Type-IIa receptor protein tyrosine phosphatases (RPTPs) and neurexins are the two major presynaptic organizers. In mammals, the type-IIa RPTPs have three members, PTPδ, PTPσ, and LAR. These members possess a large extracellular domain (ECD) consisting of three immunoglobulin-like (Ig) domains and four to eight fibronectin type-III (Fn) domains, followed by a single transmembrane helix and a cytoplasmic domain harboring two protein tyrosine phosphatase (PTP) domains: the first PTP domain is active, while the second domain is inactive. SALM family proteins have five isoforms (SALM1–SALM5). Their ECDs share the same domain organization consisting of a leucine-rich repeat (LRR) domain, an Ig domain and an Fn domain with 35% amino-acid sequence identity. We determined the crystal structures of apo-SALM5 (LRR–Ig), and PTPδ (Ig1–Ig3)–SALM2 (LRR–Ig) and PTPδ (Ig1–Fn1)–SALM5 (LRR–Ig) complexes at 3.08, 3.16, and 4.18 Å resolutions, respectively.

In the apo-SALM5 structure, the electron density of the Ig domain was mostly invisible, probably owing to the structural disorder. The electron densities of the Ig domains of SALM2 and SALM5 became relatively clear upon binding to PTPδ, suggesting that the Ig domains of SALM2 and SALM5 were partly stabilized by the interaction with PTPδ. The LRR domains of SALM2 and SALM5 are composed of eight parallel β-strands flanked by the N- and C-terminal caps. The Ig domains of SALM2 and SALM5 are positioned on the convex surface of the LRR domain and stabilized by a disulfide bond tethering the C-terminal cap and the linker connecting the LRR and Ig domains. Furthermore, in the apo-SALM5 crystal, a similar dimer-like interaction was also observed between two adjacent molecules related by crystallographic symmetry. We therefore tested the possibility of homodimer formation of SALM2 and SALM5 LRR–Ig molecules in solution by size-exclusion chromatography coupled with multi-angle laser light scattering (SEC-MALS). The theoretical molar masses of the monomeric SALM2 and SALM5 LRR–Ig-His6 molecules are 40.2 and 41.2 kDa, whereas the molar masses of the SALM2 and SALM5 LRR–Ig-His6 molecules determined by SEC-MALS are 77.0 and 77.1 kDa, respectively, indicating that both SALM2 and SALM5 form homodimers in solution. To evaluate the importance of the residues involved in hydrogen bonding in the central dimer interface, the N158A and Q134N mutants of SALM5 were analyzed by SEC-MALS. The majorities of the N158A and Q134N mutants behaved as monomers with the determined molar masses of 55.8 and 49.1 kDa, respectively. This result indicates that the hydrogen bonds in the central region of the dimer interface are critical for the dimer formation of SALM5 and also confirms the dimerization property of SALM5 in solution.

> QICPKRCVCQILSPNLATLCAKKGLLFVPPNIDRRTVELRLADNFVTNIKRKDFANMTSLVDLTLSRNTISFITPHAFADLRNLRALHLNSNRLTKITNDMFSGLSNLHHLILNNNQLTLISSTAFDDVFALEELDLSYNNLETIPWDAVEKMVSLHTLSLDHNMIDNIPKGTFSHLHKMTRLDVTSNKLQKLPPDPLFQRAQVLATSGIISPSTFALSFGGNPLHCNCELLWLRRLSREDDLETCASPPLLTGRYFWSIPEEEFLCEPPLITRHTHEMRVLEGQRATLRCKARGDPEPAIHWISPEGKLISNATRSLVYDNGTLDILITTVKDTGAFTCIASNPAGEATQIVDLHIIKLPHHHHHH> MAQHPPYCRNQPGKCQIPLRDLFDRAVVLSHYIHNLSSEMFSEFDKRYTHGRGFITKAINSCHTSSLATPEDKEQAQQMNQKDFLSLIVSILRSWNEPLYHLVTEVRGMQEAPEAILSKAVEIEEQTKRLLEGMELIVSQVHPETKENEIYPVWSGLPSLQMADEESRLSAYYNLLHCLRRDSHKIDNYLKLLKCRIIHNNNC;>MQSPPGKPEIHKCRSPDKETFTCWWNPGTDGGLPTNYSLTYSKEGEKTTYECPDYKTSGPNSCFFSKQYTSIWKIYIITVNA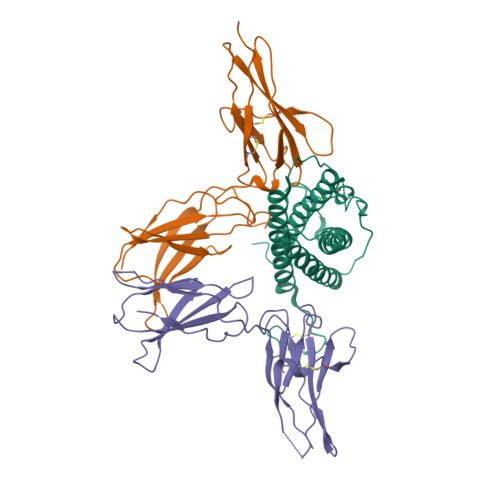TNQMGSSSSDPLYVDVTYIVEPEPPRNLTLEVKQLKDKKTYLWVKWSPPTITDVKTGWFTMEYEIRLKPEEAEEWEIHFTGHQTQFKVFDLYPGQKYLVQTRCKPDHGYWSRWSQESSVEMPNDFTLKDRSRSHHHHHH[2x]> ETKFVQALFDFNPQESGELAFKRGDV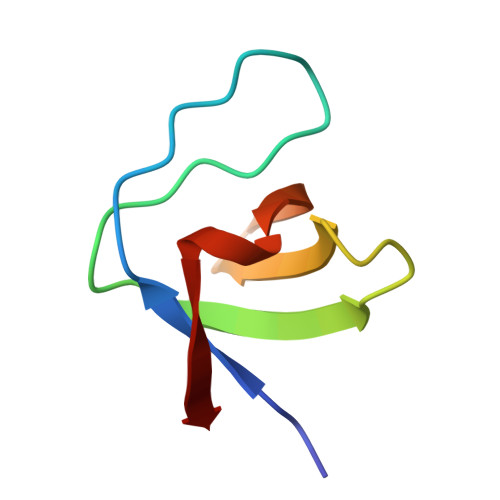ITLINKDDPNWWEGQLNNRRGIFPSNYVCPYN> ASSFEWFGSNESGAEFGSGNIPGVEGTDYTFPNTTAIQILIDAGMNIFRVPFLMERMIPTEMTGSLDTAYFEGYSEVINYITGKGAHAVVDPHNFGRYYGTPISSTSDFQTFWSTLASQFKSNDLVIFDTNNEYHDMDE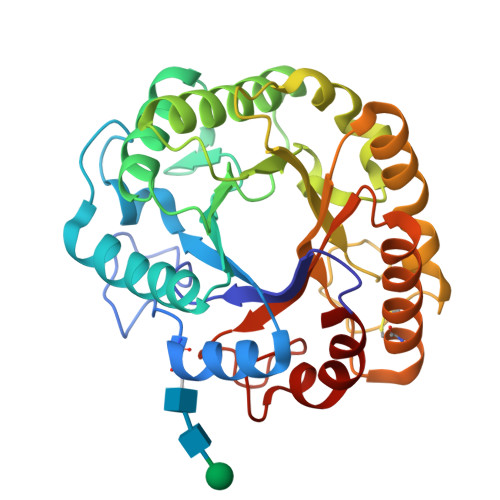SVVVALNQAAIDGIRDAGATTQYIFVEGNAYSGAWTWTTYNTAMVNLTDPSDLIVYEMHQYLDSDGSGTSDQCVSSTVGQERVVDATTWLQSNGKLGILGEFAGGANSVCEEAVEGMLDYLAENSDVWLGASWWSAGPWWQDYIYSMEPPNGIAYESYLSILETYF> NSKDSIVNDDDDSTSEVDAIPDSTNPSGSFPSVEYDVFLSFRGPDTRKQFTDFLYHFLCYYKIHTFRDDDELRKGKEIGPNLLRAIDQSKIYVPIISSGYADSKWCLMELAEIVRRQEEDPRRIILPIFYMVDPSDVRHQTGCYKKAFRKHANKFDGQTIQNWKDALKKVGDLKG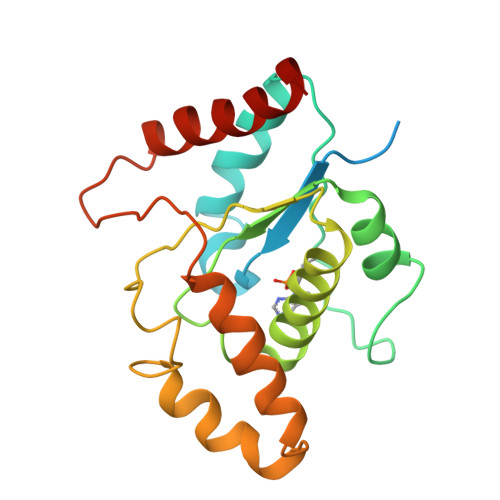WHIGKDDEQGAIADKVSADIWSHISKENL> GPVDKAGTTDNDNSQTDKTGPFSGLKFKQNSFLSTVPSVTNMHSMHFDARETFLGVIRKALEPDTSTPFPVRRAFDGLRAEILPNDTIKSAALKAQCSDIDKHPELKAKMETLKEVITHHPQKEKLAEIALQFAREAGLTRLKGETDYVLSNVLD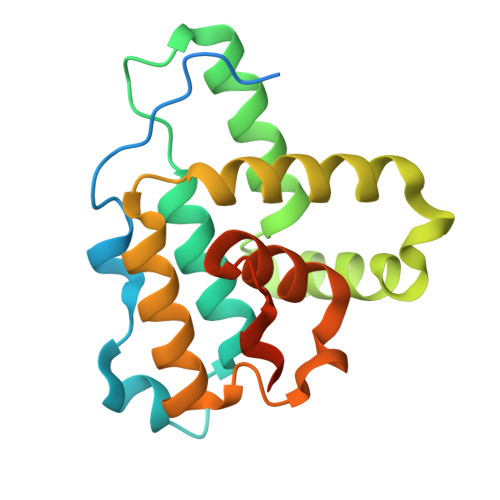GLIGDGSWRAGPAYESYLNKPG>MGSSHHHHHHSSGLVPRGSHMSNQNAPTPPPTEVIQLDWWKNCVLYQIYPRSFKDSDGDGIGDLKGIISELKHFVDAGVDAIWMSPIFESPMVDFGYDISNFYDIHYEYGTMEDFEELLDKAHELGLKVLLDFVPNHASNESEYFIKSEAREPGYENFFIWADPLPNPENPGVRLPPSNWVSQFGGSAWEWSEKRQQYYLHQFAIQQVDFDFRNPAVKQEMFNIMKFWLDKGADGFRLNALPYLIEADPADHEGRYPDDPLSGLTQFESHQLGYTIPLYTKDLIELYDVVYEWREFLDEYNKNHGGDTRVVFSEGYANVSMTMLYYGNEDGAIGAHFPFNFDFITDLSSKSNARDFVYIILRWLTYMPYGGIPNWVFGNHDNNRMPTRFRHDMVDGLNIINMLLPGVAVTYQGEEIGMRDGYVSWEDTVDIEACNRGDPDTYHLYSRDPARTPYHWDNSTSAGFSTSTNTWLPVAEDYQEINLAKQKETARSHFKNYQALTKLRKQATLSHGEYD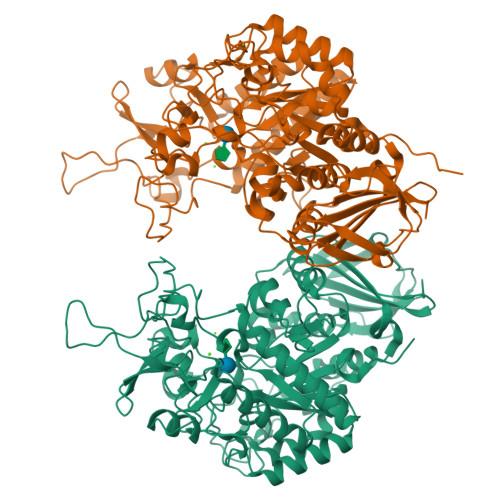IRALSDRTFYLVRSLPTHDTYVLLFNVSERRDTVDLGRVPHLTLPATVYVSSIHSARLAGHEITSSQLSLEAGEALVLKAQPI[2x]>[4x]GPGRAPPSPDLRADEPKTPCLVGGAHAFILKISSFCGLAPLRFEPRSQEYAVTISKGKCFYSYILVTFLVICTIYGLVAEIGVGVEKSVRMSSRMSQVVSACDILVVAVTAGVGVYGAPARMRTMLSYMENIVAVDRELGRHHSAATERKLCALLLLILLSFTILLVDDFCFYAMQAGKTGRQWEIVTNYAGFYFLWYIVMVLELQFAFTALSLRARLKLFNEALNVTASQVCKPVKKPKNSQLSVYATSVRPVSCKRENVIVETIRVRDKDDAFVMMKTADGVPCLQVPPCEAVGRLSRMRCTLCEVTRHIADGYGLPLVIILMSTLLHLIVTPYFLIMEIIVSTHRLHFLVLQFLWCTTHLIRMLVVVEPCHYTIREGKRTEDILCRLMTLAPHGGVLSSRLEVLSRLLMLQNISYSPLGMCTLDRPLMVTVLGAVTTYLVILIQFQRYDS

Insects, instead, rely on a distinct family of sweet gustatory receptors, which are tetrameric ligand-gated cation channels. An extreme example of sugar specialization occurs in a conserved subfamily of gustatory receptors founded by Drosophila melanogaster Gr43a (DmGr43a), whose members are selectively activated only by the monosaccharide d-fructose, providing a unique opportunity to investigate how specificity for a single sugar is achieved. Here we investigate the structural basis of sugar discrimination by Gr9 (BmGr9), the silk moth B. mori orthologue of DmGr43a. Our results thus indicate that receptor tuning in BmGr9 arises from two distinct but complementary mechanisms: the stereoelectronic characteristics of the ligand-binding pocket; and the engagement of an allosteric process required to activate the channel.

To gain insight into the mechanism of receptor activation, we also determined the structure of BmGr9 in the absence of ligand. We resolved a map of similar quality as the fructose-bound BmGr9 but with the extracellular hydrophobic gate closed, consistent with the absence of any density in the ligand-binding pocket. In the unbound structure, Phe444 side chains from each subunit face the centre of the ion-conducting pore, erecting a hydrophobic barrier that constricts the pore diameter and prevents ion passage, similar to the gate observed in olfactory receptors. In the closed state, Gln443 hydrogen bonds with Gln445 from a neighbouring subunit. In the absence of a ligand, the vestibule connecting the pocket to the extracellular surface is approximately 8 Å wide, large enough for sugar molecules to access the bottom of the pocket freely. In the closed state, Tyr332 and Phe333 are exposed to the membrane interior through a gap between the S7b and S2 helices, where additional columnar lipid or detergent density is observed in the structure of unbound BmGr9. Nearby, Arg90 in S2 reaches across the gap between subunits to interact with carboxy-terminal carbonyls of S5 in the absence of ligand.> XIWLAQGARRLGDEIN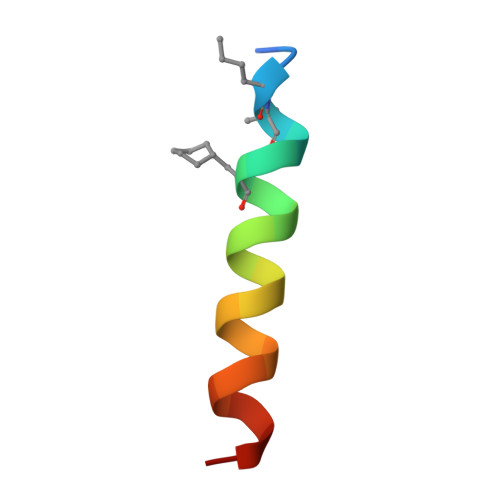AYYARRX>[5x]GAMGQTSTRWTPTTEQIKILKELYYNNAIRSPTADQIQKITARLRQFGKIEGKNVFYWFQNHKARERQKKRFNGGS

The HD transcription factor WUS plays key roles for plant development with at least four distinct and essential subfunctions: Firstly, regulation of stem cell identity in the shoot apical meristem (SAM), where it is required for non cell-autonomous induction and maintenance of stem cell fate via stimulation of cytokinin and suppression of auxin signaling. Consistent with a broad functional portfolio, WUS has been shown to bind to a diverse set of DNA motifs in the regulatory regions of downstream genes involved in SAM development and signaling processes. Here, we have combined molecular, biochemical, and structural approaches to address how the WUS-HD recognizes specific DNA target sites. We find that the DNA-binding preferences of WUS-HD depend on appropriately arranged sequence motifs in a direct tandem repeat and that homodimerization is one of the key determinants to achieve high sequence specificity.

To elucidate the structural basis for these differential interactions, we solved crystal structures of WUS-HD bound to TAAT, G-Box and TGAA repeat probes to resolutions of 2.8, 2.7 and 1.6 Å, respectively. Interestingly, in the case of G-Box and TAAT, one of the two protein–DNA complexes in the asymmetric unit contained an additional bound HD, whereas both TGAA structures only included two HDs per DNA. In both cases, this additional molecule inserted its C-terminal recognition helix into a major groove of the DNA on the complementary strand of one of the prevalent recognition motifs, but did not make contact to the other two protein molecules. In the G-Box structure, this extra HD (Fig. 2d teal) was stabilized by crystal contacts from the neighboring complex and thus likely represents a crystallization artifact. Bound to the G-Box probe, the two monomers were positioned head-to-head on the same side of the DNA and had almost identical binding features, probably due to the palindromic nature of the DNA recognition sequence and the negligible interaction between them. The binding of the “atypical” Extradenticle (Exd) HD (PDB code 2R5Y30) to a core TGAT motif, although very similar in sequence, also shows some differences in the hydrogen bond pattern compared to WUS-HD bound to the G-Box probe. Notably, the conserved R38 of the N-terminal arm in our structure neither contacted the −1 nor the −2 position of the sense-strand. However, the guanine at position −1 was specified by R94 in the C-terminal recognition helix, following the usual mechanism for HDs contacting atypical recognition motifs. In the G-Box crystal structure, Y86 formed Van der Waals interactions with thymine of the +1 position of the TGAT motif.>NEQLAKQKGCMACHDLKAGGGKKVGPAYADVAKKYAGRKDAVDYLAGKIKKGGSGVWGSVPMPPQNVTDAEAKQL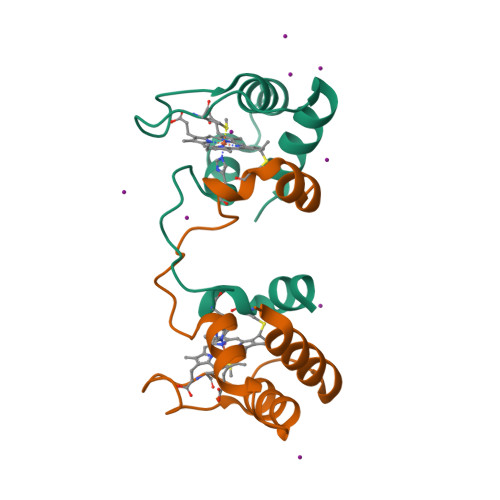AQWILSIK[4x]>[4x]MPQLHYVPYDTPVEDVMRILKESGTLVIRNFLDQNTVQKVQDEVDDYVRNWNPGPKYNHDIKNVGSKTKQPSNLSLMSKTYRCEVLNHPWMHAICERMFGPTYGDYWFNGGAILHLEPGENTQPIHQDHVFYQISKWRRPTDPDLTINFTMALTEFTVENGGTRVCPGSHLWENGHASPAEEDMVPVLMQPGDALILPGSMWHSAGA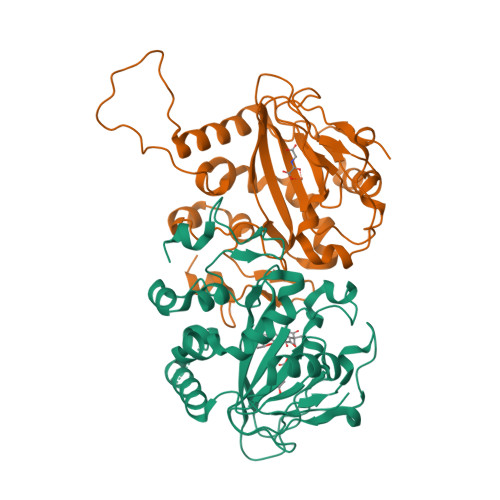NRTSEYRRGFATSFHPCHFTPIESHHHLPREMVEEMTPLVQKMLGFRTLNLHNNVKVWKAGEGNLEDATGLKSVAAKLAAALEHHHHHH> MVILGVGYFLLGLILLYYGSDWFVLGSERIARHFNVSNFVIGATVMAIGTSLPEILTSAYASYMHAPGISIGNAIGSCICNIGLVLGLSAIISPIIVDKNLQKNILVYLLFVIFAAVIGIDGFSWIDGVVLLILFIIYLRWTVKNGSAEIEENNDKNNPSVVFSLVLLIIGLIGVLVGAELFVDGAKKIALALDISDKVIGFTLVAFGTSLPELMVSLA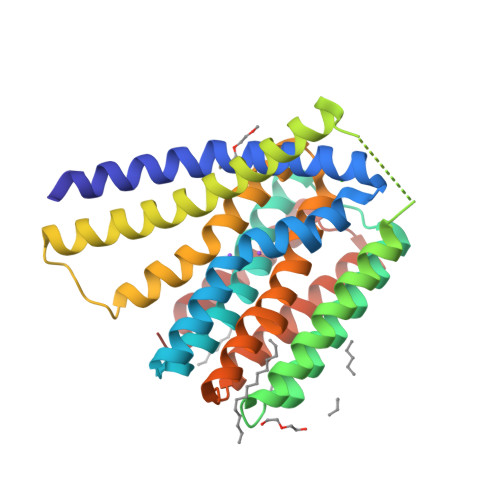AAKRNLGGMVLGNVIGSNIADIGGALAVGSLFMHLPAENVQMAVLVIMSLLLYLFAKYSKIGRWQGILFLALYIIAIASLRM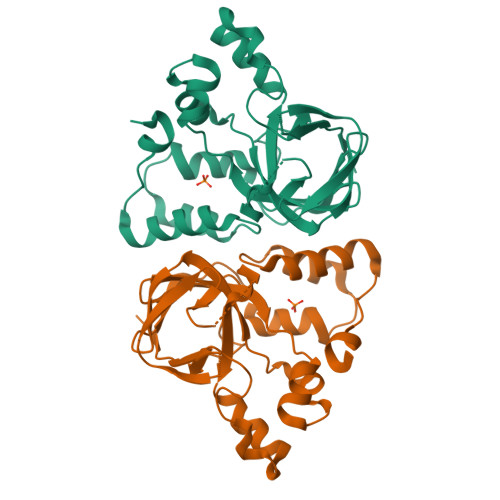>GSAKDPMRYPVDVYTGKIQAYPEGKPSAIAKIQVDGELMLTELGLEGDEQAEKKVHGGPDRALCHYPREHYLYWAREFPEQAELFVAPAFGENLSTDGLTESNVYMGDIFRWGEALIQVSQPRSPCYKLNYHFDISDIAQLMQNTGKVGWLYSVIAPGKVSADAPLELVSRVSDVTVQEAAAIAWHMPFDDDQYHRLLSAAGLSKSWTRTMQKRRLSGKIEDFSRRLWGK[2x]Beta(β)-lactamases are bacterial enzymes that provide multi-drug resistance to β-lactam antibiotics. Mtb β-lactamase (BlaC) is a broad-spectrum Ambler class A3 β-lactamase capable of hydrolyzing all classes of β-lactam antibiotics used for the treatment of tuberculosis. Sulbactam (SUB), clavulanate and tazobactam, all β-lactam based suicide inhibitors, irreversibly bind to β-lactamases and block their activity. Here, we report in atomic detail (between 2.2 and 2.7 Å resolution) by room-temperature, time-resolved crystallography with millisecond time-resolution (with timepoints between 3 ms and 700 ms) how the Mycobacterium tuberculosis enzyme BlaC is inhibited by sulbactam (SUB).

At 3, 6, and 15 ms, the DED features near the active site of subunit A are weak. Substantial displacements of the residues flanking the active site are observed. Particularly, the long-side chain residues such as Gln112B and Arg173 (called guardian residues) move outward from the active site before relaxing back to their original positions. Next to these residues at 3 ms, almost 10 Å away from Ser70, there are positive densities that are spatially more spread out than that of water. An SUB molecule can be placed in the electron density. However, refinement of the SUB is difficult (see Supplementary Fig. 1a for an explanation). Nevertheless, contrary to expectations based on the size of the SUB, no electron density is present at the earliest time points. This can be explained by the smaller second-order binding coefficient, kncov (1.5 mM−1 s−1 for SUB compared to 3.2 mM−1 s−1 for CEF), which prevents the accumulation of electron density at earlier times.

>GADLADRFAELERRYDARLGVYVPATGTTAAIEYRADERFAFCSTFKAPLVAAVLHQNPLTHLDKLITYTSDDIRSISPVAQQHVQTGMTIGQLCDAAIRYSDGTAANLLLADLGGPGGGTAAFTGYLRSLGDTVSRLDAEEPELNRDPPGDERDTTTPHAIALVLQQLVLGNALPPDKRALLTDWMARNTTGAKRIRAGFPADWKVIDKTGTGDYGRANDIAVVWSPTGVPYVVAVMSDRAGGGYDAEPREALLAEAATCVAGVLA[4x]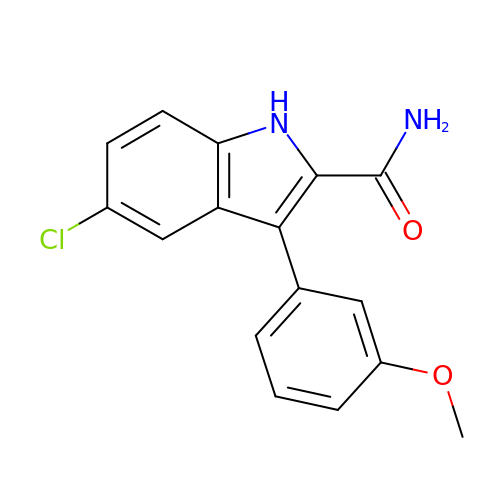5-chloranyl-3-(3-methoxyphenyl)-1~{H}-indole-2-carboxamide | C16 H13 Cl N2 O2 | INZGVMONFMTZEK-UHFFFAOYSA-N>MDTGVTSPRVLVVDDDSDVLASLERGLRLSGFEVATAVDGAEALRSATENRPDAIVLDINMPVLDGVSVVTALRAMDNDVPVCVLSARSSVDDRVAGLEAGADDYLVKPFVLAELVARVKALLRRRGSTATSSSETITVGPLEVDIPGRRARVNGVDVDLTKREFDLLAVLAEHKTAVLSRAQLLELVWGYDFAADTNVVDVFIGYLRRKLEAGGGPRLL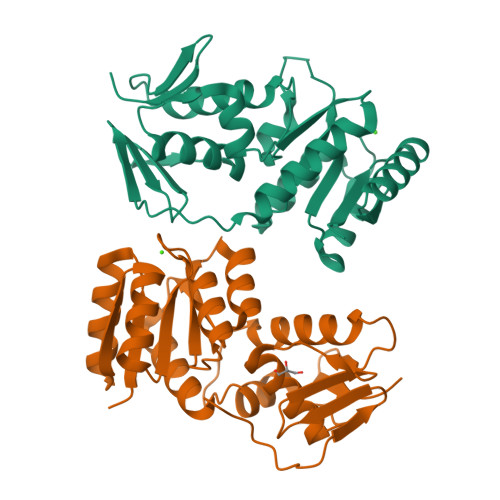HTVRGVGFVLRMQ[2x]> MVKVDLESKRYGEKLKEVFLMLDNNVVECIKEITESSRNGKLVFFVGAGVSTLSDYPQWWRLVDKYHEELYGSPKKGNYSSDEYLRIPQIFYNVKGEMAFDGILKDFFQVDKPTNPIHDKILAMNPAHVITTNYDNLIDTACWKRGKYFSVISAEEDVANATSSRYLLKVAGDFRKGFKGENVVLKEDDYLNYDQNYPLISNLMKTIIATHTIVFIGYGLGDYNINMLLNWVRKLQKDSFHKPFFIRTDPSPIENETLIYYENKGLRIIDAASLIDSNEYDYLERYSAVMDLLIESQENKFITKDDEVIDYIYGKISPLFALQYIRKIDLKHVFEYDYHFEVNGTVVRHKNKGFGYMERFFELKESCDERSKLSKKQYERFNALFNFFEKNGVICMAKDAGTLNTSIEINSLAYHGKYDVMKKFIEEQSVSIEDDYKKAFFLACLGRWEESYDLYSNIILNSIDESNGCVYYLSQINRYRIYQSITQAVTQFNGLGLLTFGRHYKPFTDEFLARIEREMTNFNIDDLFNGMPFEFQKKYKILEFLSDNQFLYDDTVKLFELTNKVRSEMSEGSYSFGMSSDIVVLLRLYDNLRFLYENCLWSVSFHEFHQYIRNSMSLLIEKAEYERTRDIDELGFSFFGKKSGFFMEYYDFVNISRHFKIDDIKNLERSCSIDKIRFGEQEKIEEYLVGIAEEITKQFSANGMNVVFYTQFISEAKAALYFAKYVKLSEEGLGKIVKALLFYFPERDLDIGKRYVWLERLTKCNELPKSIISIIDDFLVLQAEKHIDQNYSEVSSNGLYSRDYGALIKHFEKNFISKRLSEITLCLTQDKQKQIDFLFKLLPLLSTNAKSHLLS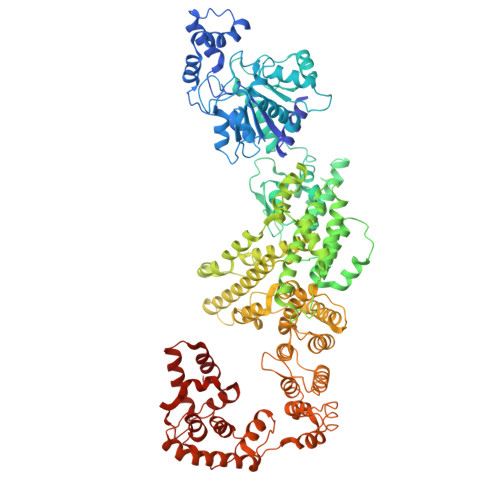FKSVENINDLMNGIRIGLIDEFTPEHEELIIEYLETRKVNYIVEKEKGIQTFSSNDYMSTFGIWYFLEEINNSKMEEFIGMDDQYDFFVDPENFDYKKFIPSWLKNYNDKLLGKIAGNKHMKHHVIEVLKERVKNSNDKRYLEILMNYFI>[5x]DTTQPALLRLSDHLLANYKKGVRPVRDWRKP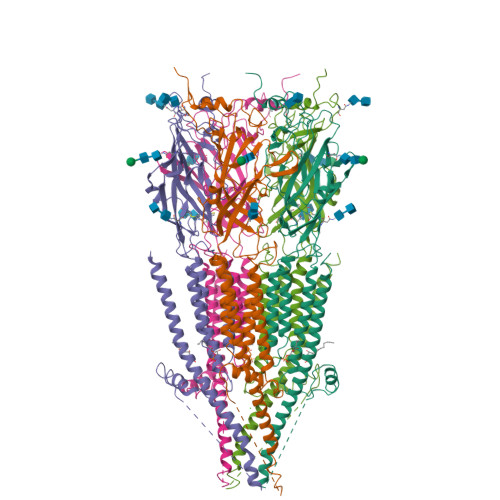TTVSIDVIMYAILNVDEKNQVLTTYIWYRQYWTDEFLQWTPEDFDNVTKLSIPTDSIWVPDILINEFVDVGKSPNIPYVYVHHRGEVQNYKPLQLVTACSLDIYNFPFDVQNCSLTFTSWLHTIQDINITLWRSPEEVRSDKSIFINQGEWELLEVFPQFKEFSIDISNSYAEMKFYVIIRRRPLFYAVSLLLPSIFLMVVDIVGFCLPPDSGERVSFKITLLLGYSVFLIIVSDTLPATAIGTPLIGVYFVVCMALLVISLAETIFIVRLVHKQDLQRPVPDWLRHLVLDRIAWILCLGEQPMAHRPPATFQANKTDDCSGSDLLPAMGNHCSHVGGPQDLEKTPRGRGSPLPPPREASLAVRGLLQELSSIRHFLEKRDEMREVARDWLRVGYVLDRLLFRIYLLAVLAYSITLVTLWSIWHYS>MKIARVCGTVTSTQKEDTLTGVKFLVLQYLGEDGEFLPDYEVAADTVGAGQDEWVLVSRGSAA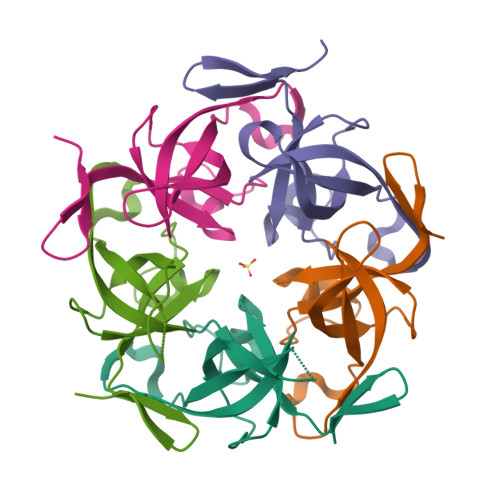RHIINGTDKPIDAAVVAIIDTVSRDNYLLYSKRTQY[5x]>MSHYRSNVRDQVFNLFEVLGVDKALGHGEFSDVDVDTARDMLAEVSRLAEGPVAESFVEGDRNPPVFDPKTHSVMLPESFKKSVNAMLEAGWDKVGIDEALGGMPMPKAVVWALHEHILGANPAVWMYAGGAGFAQILYHLGTEEQKKWAVLAAERGWGSTMVLTEPDAGSDVGAARTKAVQQADGSWHIDGVKRFITSGDSGDLFENIFHLVLARPEGAGPGTKGLSLYFVPKFLFDVETGEPGERNGVFVTNVEHKMGLKVSATCELAFGQHGVPAKGWLVGEVHNGIAQMFEVIEQARMMVGTKAIATLSTGYLNALQYAKSRVQGADLTQMTDKTAPRVTITHHPDVRRSLMTQKAYAEGLRALYLYTATFQDAAVAEVVHGVDAKLAVKVNDLMLPVVKGVGSEQAYAKLTESLQTLGGSGFLQDYPIEQYIRDAKIDSLYAGTTAIQAQDFFFRKIVRDKGVALAHVSGQIQEFVDSGAGNGRLKTERALLAKALTDVQGMAAALTGYLMAAQQDVTSLYKVGLGSVRFLMSVGDLIIGWLLQRQAAVAVAALDAGATGDERSFYEGKVAVASFFAKNFLPLLTSTREVIE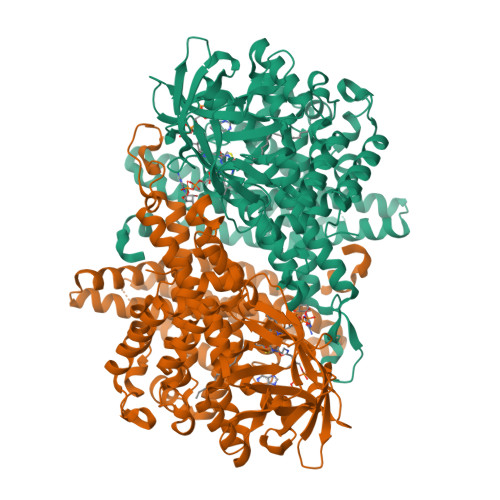TLDNDIMELDEAAF[2x]> GASGDLYEVERIVDKRKNKKGKWEYLIRWKGYGSTEDTWEPEH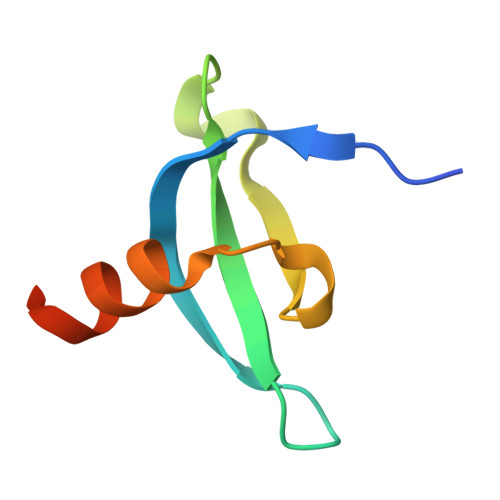HLLHCEEFIDEFNGLHMSKDK>[2x]MSQNNPLRALLDKQDILLLDGAMATELEARGCNLADSLWSAKVLVENPELIREVHLDYYRAGAQCA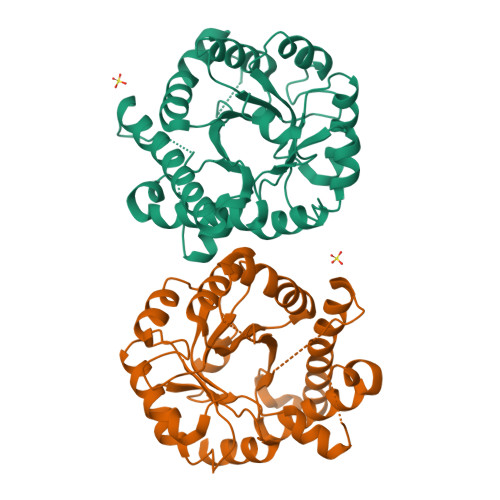ITASYQATPAGFAARGLDEAQSKALIGKSVELARKAREAYLAENPQAGTLLVAGSVGPYGAYLADGSEYRGDYHCSVEAFQAFHRPRVEALLDAGADLLACETLPNFSEIEALAELLTAYPRARAWFSFTLRDSEHLSDGTPLRDVVALLAGYPQVVALGINCIALENTTAALQHLHGLTVLPLVVYPNSGEHYDAVSKTWHHHGEHCAQLADYLPQWQAAGARLIGGCCRTTPADIAALKARS> TQLDIVIVLDGSNSIYPWDSVTAFLNDLLKRMDIGPKQTQVGIVQYGENVTHEFNLNKYSSTEEVLVAAKKIVQRGGAQTMTALGTDTARKEAFTEARG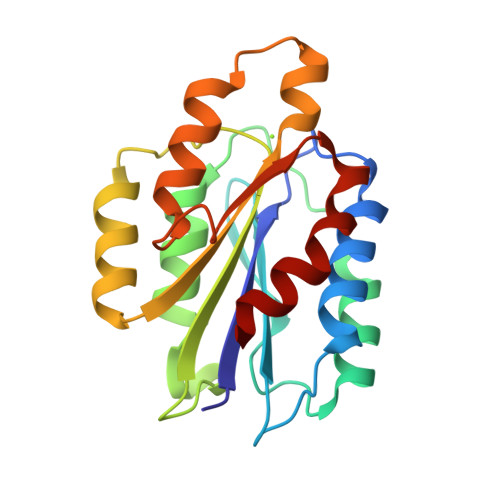ARRGVKKVMVIVTDGESHDNHRLKKVIQDCEDENIQRFSIAILGSYNRGNLSTEKFVEEIKSIASEPTEKHFFNVSDELALVTIVKTLGERIFA>[2x]FACKTANGTAIPIGGGSANVYVNLAPVVNVGQNLVVDLSTQIFCHNDYPETITDYVTLQRGSAYGGVLSNFSGTVKYSGSSYPFPTTSETPRVVYNSRTDKPWPVALYLTPVSSAGGVA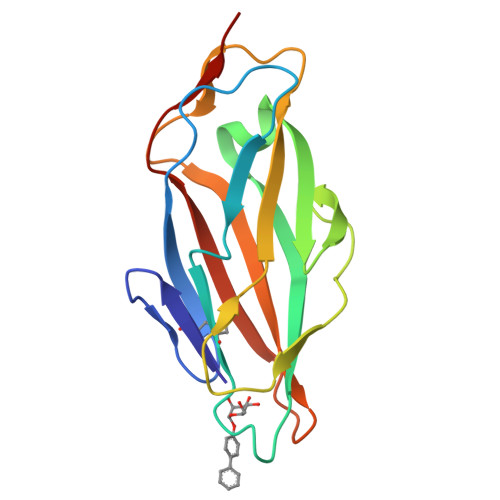IKAGSLIAVLILRQTNNYNSDDFQFVWNIYANNDVVVPTGL>[4x]HHHHHHASMDKNIIIGAMTALITPFKNGKVDEQSYARLIKRQIENGIDAVVPVGTTGESATLTHEEHRTCIEIAVETCKGTKVKVLAGAGSNATHEAVGLAKFAKEHGADGILSVAPYYNKPTQQGLYEHYKAIAQSVDIPVLLYNVPGRTGCEISTDTIIKLFRDCENIYGVKEASGNIDKCVDLLAHEPRMMLISGEDAINYPILSNGGKGVISVTSN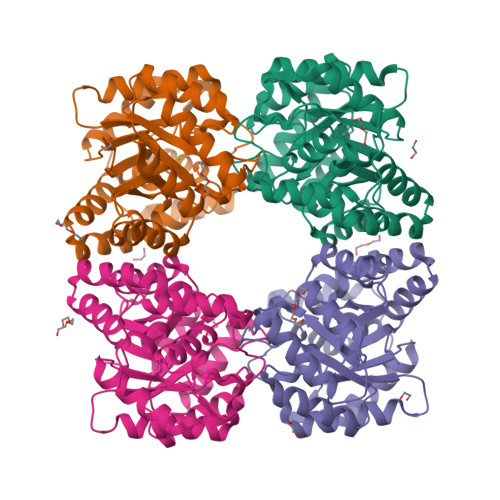LLPDMISALTHFALDENYKEAKKINDELYNINKILFCESNPIPIKTAMYLAGLIESLEFRLPLCSPSKENFAKIEEVMKKYKIKGF>[2x]MKIKGVNLGNWLVLEKWMSSAIWEGTDAEDEYYLPRGLDSKVYEARIKMHRAEYISERDFARIKAMGFNSVRIPIPYFIYGDRAPFIGCIDELDRAFSWAEKYDLKILIDLHTVPMSQNGFDNGGLSGVCKWAQIPEEVDFVLNLLEKLAKRYGKRKGLLGIEPINEPVSEEMWNDMGVQKRYPPLDKEMAEGSAPISFEWLKGFYDKAADRIL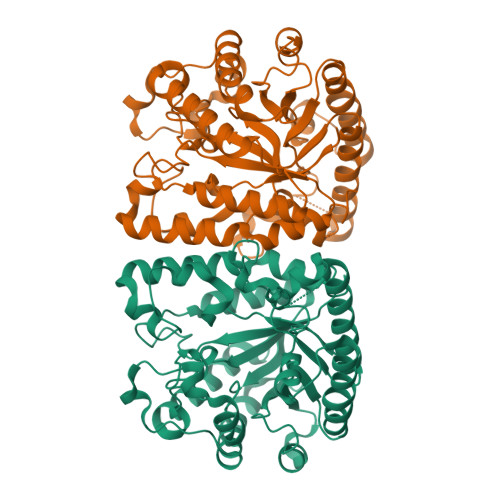PNIDDDKYIVFHDGFRLHAWEEYLTQDRYKGRVILDTHQYLMIAEMLGCEQTLEAYKTFIKEKFEDEITKVEKYVPVVVGEWCIFNSYCVGMDTKGGQSVLNGVDSSDAKGVSDEEKRKVYMELSKAQLKAWDSLSGYFYWTYKMLLDPTNQATWRGWDCWDLAKCVDEGWFPGRVA> MAEKQRQLKLQKIYKQKYIGLGDESTTREQWQRNVRNDTLNTLQGHSASLEYVSLSRGDLSIRDTRIHLLK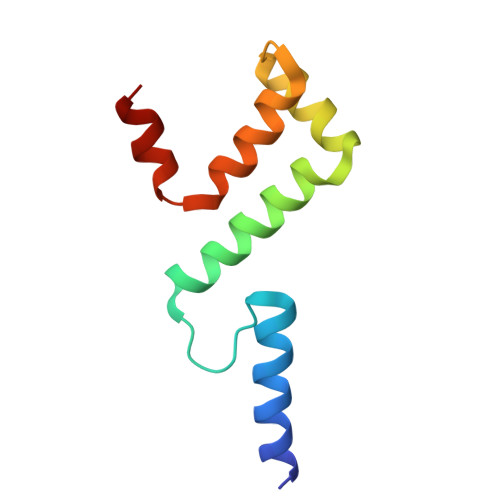SMSPGYKAYLREER>GSSGSSGSLEVSVGKATTIYAINGSSILLPCTFSSCYGFENLYFKWSYNNSETSRILIDGIVKNDKSDPKVRVKDDDRITLEGSTKEKTNNISILLSDLEFSDT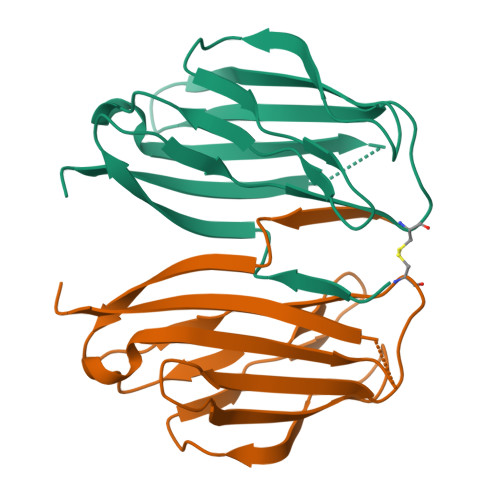GRYTCFVRNPKEKDLNNSATIFLQVVDKLEKVDN[2x]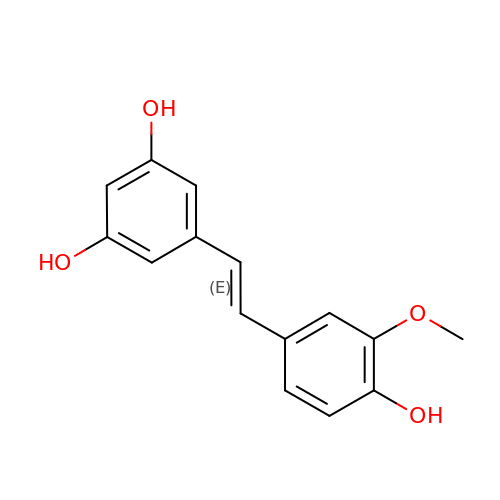5-[(~{E})-2-(3-methoxy-4-oxidanyl-phenyl)ethenyl]benzene-1,3-diol | C15 H14 O4 | ANNNBEZJTNCXHY-NSCUHMNNSA-N> LINECGAGPDLITLSE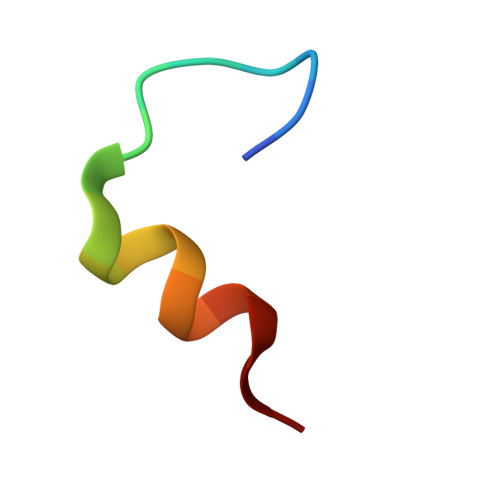QR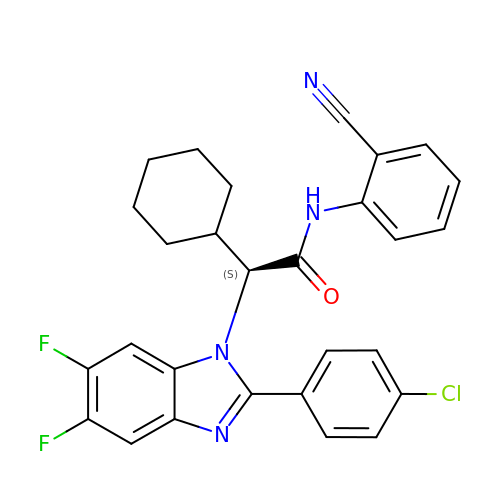(2S)-2-[2-(4-chlorophenyl)-5,6-difluoro-1H-benzimidazol-1-yl]-N-(2-cyanophenyl)-2-cyclohexylacetamide | C28 H23 Cl F2 N4 O | KQOKFDLIIQSPMA-SANMLTNESA-N>[4x]MKNLSAYEVYESPKTSGESRTEAVSEAAFESDPEVSAILVLTSSEASTLERVADLVTAHALYAAHDFCAQAQLAAAELPSRVVARLQEFAWGDMNEGHLLIKGLPQVRSLPPTPTSNVHAVAATTPMSRYQALINECVGRMIAYEAEGHGHTFQDMVPSAMSAHSQTSLGSAVELELHTEQAFSPL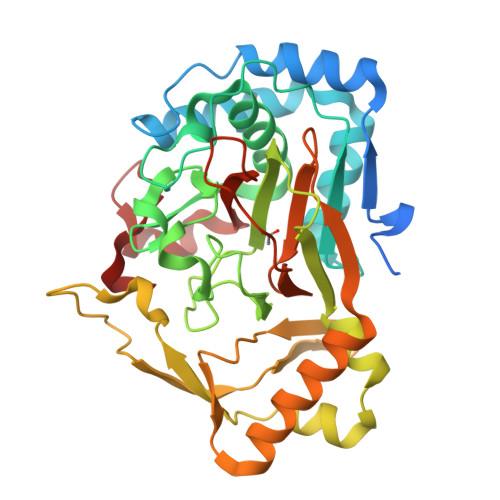RPDFVSLACLRGDPRALTYLFSARQLVATLTTQEIAMLREPMWTTTVDESFLAEGRTFLLGFERGPIPILSGADDDPFIVFDQDLMRGISAPAQELQQTVIRAYYAERVSHCLAPGEMLLIDNRRAVHGRSIFAPRFDGADRFLSRSFIVADGSRSRHARSSFGRVVSARFS5,5'-[propane-1,3-diylbis(oxy-4,1-phenylene)]bis(6-ethylpyrimidine-2,4-diamine) 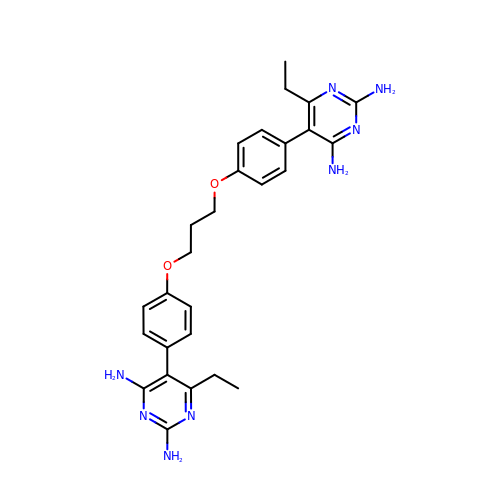| C27 H32 N8 O2 | CWKNXRKHGBGSLU-UHFFFAOYSA-N3-[(2R)-2-(dihydroxyboranyl)-2-{[(2R)-2-{[(4-ethyl-2,3-dioxo-3,4-dihydropyrazin-1(2H)-yl)carbonyl]amino}-2-(4-hydroxyphenyl)acetyl]amino}ethyl]benzoic 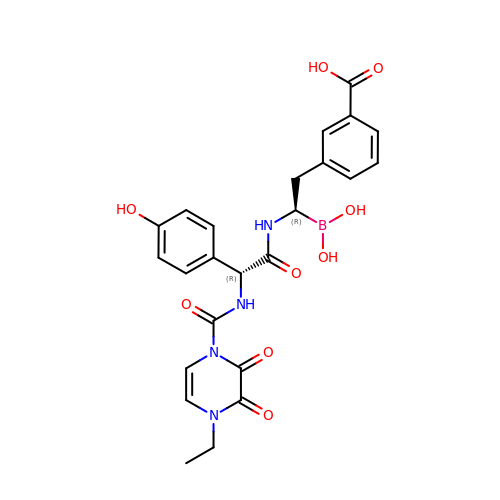acid | C24 H25 B N4 O9 | ALFFAZKBOABSLT-RBUKOAKNSA-N>[8x]XSKLLLLLIILSEALHL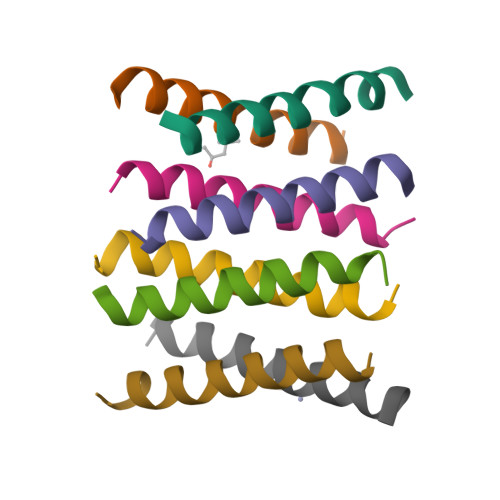AILLLIKWGX>[2x]MSDQNNRSRNEYHSNRKNEPSYELQNAHSGLFHSSNEELTNRNQRYTNQNASMGSFTPVQSLQFPEQSQQTNMLYNGDDGNNNTINDNERDIYGGFVNHHRQRPPPATAEYNDVFNTNSQQLPSEHQYNNVPSYPLPSINVIQTTPELIHNGSQTMATPIERPFFNENDYYYNNRNSRTSPSIASSSDGYADQEARPILEQPNNNMNSGNIPQYHDQPFGYNNGYHGLQAKDYYDDPEGGYIDQRGDDYQINSYLGRNGEMVDPYDYENSLRHMTPMERREYLHDDSRPVNDGKEELDSVKSGYSHRDLGEYDKDDFSRDDEYDDLNTIDKLQFQANGVPASSSVSSIGSKESDIIVSNDNLTANRALKRSGTEIRKFKLWNGNFVFDSPISKTLLDQYATTTENANTLPNEFKFMRYQAVTCEPNQLAEKNFTVRQLKYLTPRETELMLVVTMYNEDHILLGRTLKGIMDNVKYMVKKKNSSTWGPDAWKKIVVCIISDGRSKINERSLALLSSLGCYQDGFAKDEINEKKVAMHVYEHTTMINITNISESEVSLECNQGTVPIQLLFCLKEQNQKKINSHRWAFEGFAELLRPNIVTLLDAGTMPGKDSIYQLWREFRNPNVGGACGEIRTDLGKRFVKLLNPLVASQNFEYKMSNILDKTTESNFGFITVLPGAFSAYRFEAVRGQPLQKYFYGEIMENEGFHFFSSNMYLAEDRILCFEVVTKKNCNWILKYCRSSYASTDVPERVPEFILQRRRWLNGSFFASVYSFCHFYRVWSSGHNIGRKLLLTVEFFYLFFNTLISWFSLSSFFLVFRILTVSIALAYHSAFNVLSVIFLWLYGICTLSTFILSLGNKPKSTEKFYVLTCVIFAVMMIYMIFCSIFMSVKSFQNIL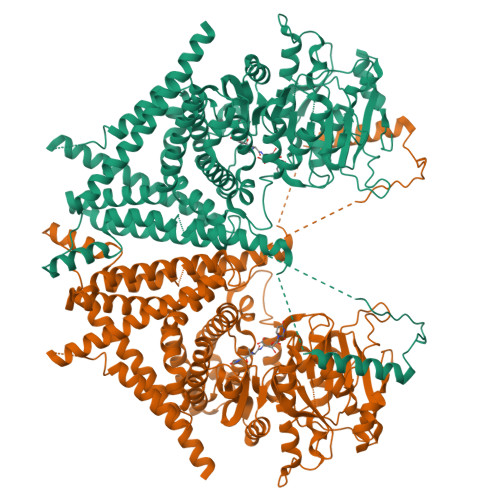KNDTISFEGLITTEAFRDIVISLGSTYCLYLISSIIYLQPWHMLTSFIQYILLSPSYINVLNIYAFCNVHDLSWGTKGAMANPLGKINTTEDGTFKMEVLVSSSEIQANYDKYLKVLNDFDPKSESRPTEPSYDEKKTGYYANVRSLVIIFWVITNFIIVAVVLETGGIADYIAMKSISTDDTLETAKKAEIPLMTSKASIYFNVILWLVALSALIRFIGCSIYMIVRFFKKVTFR>MFKNLIWLKEVDSTQERLKEWNVSYGTALVADRQTKGRGGLGRKWLSQEGGLYFSFLLNPKEFENLLQLPLVLGLSVSEALEEITEIPFSLKWPNDVYFQEKKVSGVLRELSKDKLIVGIGINVNQREIPEEIKDRATTLYEITGKDWDRKEVLLKVLKR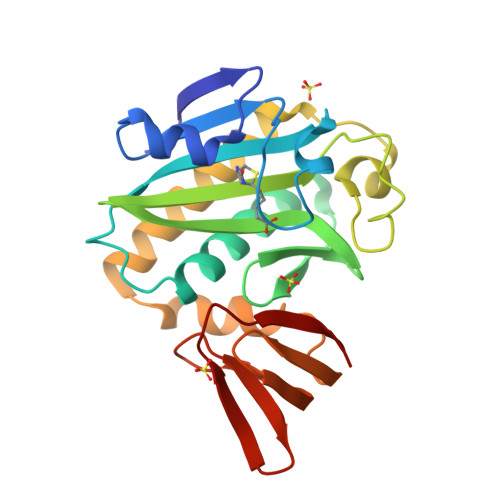ISENLKKFKEKSFKEFKGKIESKMLYLGEEVKLLGEGKITGKLVGLSEKGGALILTEEGIKEILSGEFSLRRS[2x]>MDKERIIQEFVPGKQVTLAHLIAHPGEELAKKIGVPDAGAIGIMTLTPGETAMIAGDLALKAADVHIGF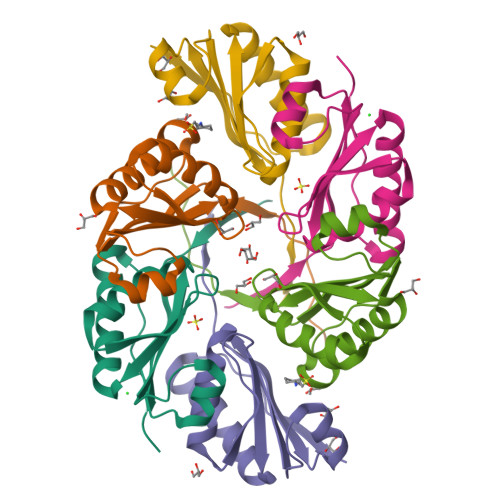LDRFSGALVIYGSVGAVEEALSQTVSGLGRLLNYTLCEMTKSLEHHHHHH[3x]> KAVLFPDGQAVGEKIFKTAGAVKSYSDAEQLCREAKGQLASPRSSAENEAVTQMVRAQEKNAYLSMND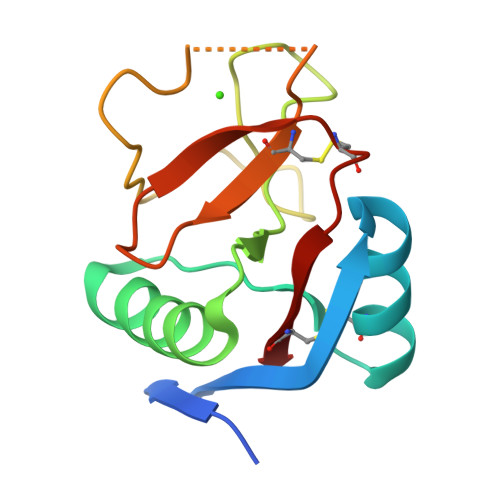ISTEGRFTYPTGEILVYSNWADGEPNNSDEGQPENCVEIFPDGKWNDVPCSKQLLVICEF>[2x]MSHHHHHHSMKTLVIAHRGDSKNVPENTIAAFKRAMELGADGIELDVQLTKDGHLVVIHDETVDRTTNGEGFVKDFTLEEIKKLDAGIKFGEKFAGERIPTL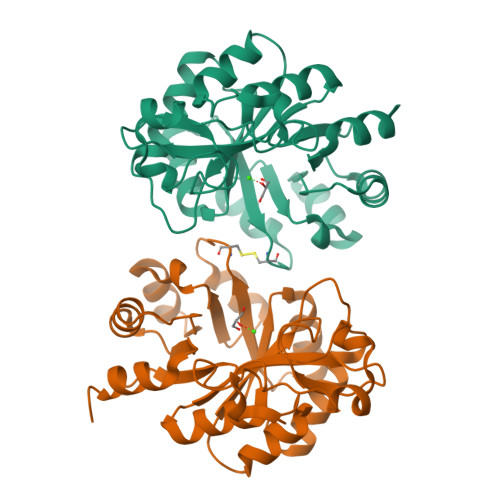YEVFELIGDKDFLVNIEIKSGIVLYPGIEEKLIKAIKEYNFEERVIISSFNHYSLRDVKKMAPHLKIGLLYQCGLVEPWHMALRMEAYSLHPFYFNIIPELVEGCKKNGVKLFPWTVDRKEDMERMIKAGVDGIITDDPETLINLVRKGG> AGQGDGSVIELGEQTVVATAQEETKQAPGVSIITAEDIAKRPPSNDLSQIIRTMPGVNLTGNSSSGQRGNNRQIDIRGMGPENTLILVDGKPVSSRNSVRYGWRGERDSRGDTNWVPADQVERIEVIRGPAAARYGNGAAGGVVNIITKQAGAETHGNLSVYSNFPQHKAEGASERMSFGLNGPLTENLSYRVYGNIAKTDSDDWDINAGHESNRTGKQAGTLPAGREGVRNKDIDGLLSWRLTPEQTLEFEAGFSRQGNIYTGDTQNTNSNNYVKQMLGHETNRMYRETYSVTHRGEWDFGSSLAYLQYEKTRNSRINEGLAGGTEGIFDPNNAGFYTATLRDLTAHGEVNLPLHLGYEQTLTLGSEWTEQKLDDPSSNTQNTEEGGSIPGLAGKNRSSSSSARIFSLFAEDNIELMPGTMLTPGLRWDHHDIVGDNWSPSLNLSHALTERVTLKAGIARAYKAPNLYQLNPDYLLYSRGAGCYGQSTSCYLRGNDGLKAETSVNKELGIEYSHDGLVAGLTYFRNDYKNKIESGLSPVDHASGGKGDYANAAIYQWENVPKAVVEGLEGTLTLPLADGLKWSNNLTYMLQSKNKETGDVLSVTPRYTLNSMLDWQATDDLSLQATVTWYGKQKPKKYDYHGDRVTGSANDQLSPYAIAGLGGTYRLSKNLSLGAGVDNLFDKRLFRAGNAQGVVGIDGAGAATYNEPGRTFYTSLTASF

In Gram-negative bacteria, Fe3+-siderophore complexes are recognised at the bacterial cell surface by highly selective outer-membrane TonB-dependent transporters (TBDTs). These transporters bind the Fe3+-siderophore complex and translocate it into the periplasm. The structures of pyoverdine, pyochelin, citrate and ferrichrome iron complexes bound to their respective transporters FpvA, FptA, FecA and FhuA showed that the ferric-siderophore complexes were bound inside the barrel adjacent to the plug domain, a position thought to be poised for translocation. Pseudomonas aeruginosa, a serious opportunistic pathogen, does not make enterobactin but does possess a TBTD outer-membrane protein PfeA, related to FepA, that binds and translocates Fe3+-enterobactin into the periplasm. PfeA has the same two domains (22-stranded β-barrel and N-terminal plug) common to the TBDTs.

We constructed four mutants R480A, Q482A, G324V and R480A-Q482A (double mutant) to validate the observed recognition site. Each of the mutant proteins was purified as described for the parent protein, and crystal structures of each were obtained. These structures were essentially identical to that of the parent protein, which confirmed that the mutations did not affect the folding of the protein. Co-complexes with Fe3+-enterobactin were obtained by soaking for the R480A and Q482A mutants. Apart from the mutation itself and an additional water molecule in R480A, the mutant complexes were essentially identical except that the B-factors of the Fe3+-enterobactin molecules were higher reflecting a bigger mobility or a partial occupancy of the ligand. Mutant Q482A showed biphasic isotherms, but with much reduced heat output and smaller K1 values. Two single-site mutations (R480A, Q482A) of interacting residues revealed weakened (but detectable) binding in ITC experiments, behaviour predicted from the structural model and consistent with a genuine-binding site. We further note that in order to form this binding site, the protein undergoes the same conformational changes for all three compounds and in Q482A and R480A mutants.> NGSSSCIEEVSVPDDNWYRIANELLSRAGIAINGSAPADIRVKNPDFFKRVLQEGSLGLGESYMDGWWECDRLDMFFSKVLRAGLENQLPHHFKDTLRIAGARLFNLQSKKRAWIVGKEHYDLGNDLFSRMLDPFMQYSCAYWKDADNLESAQQAKLKMICEKLQLKPGMRVLDIGCGWGGLAHYMASNYDVSVVGVTISAEQQKMAQERCEGLDVTILLQDYRDLNDQFDRIVSVGMFEHVGPKNYDTYFAVVDRNLKPEGIFLLHTIGSKKTDLNVDPWINKYIFPNGCLPSVRQIAQSSEPHFVMEDWHNFGADYDTTLMAWYERFLAAWPEIADNYSERFKR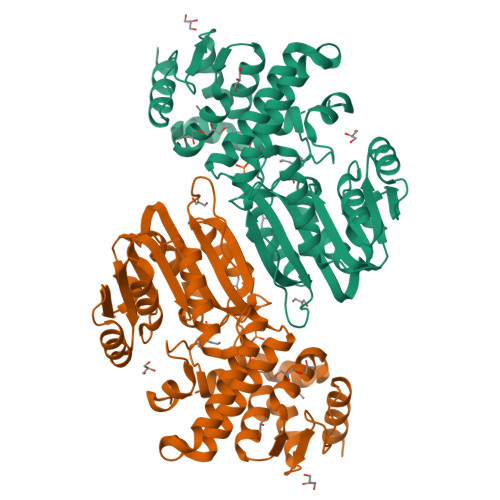MFTYYLNACAGAFRARDIQLWQVVFSRGVENGLRVAR>KSQVKIRFFTREKDELLHVQDTPMYAPISLKRYGLSEIVNHLLGSEKPVPFDFLIEGELLRTSLHDYLTKKGLSSEASLN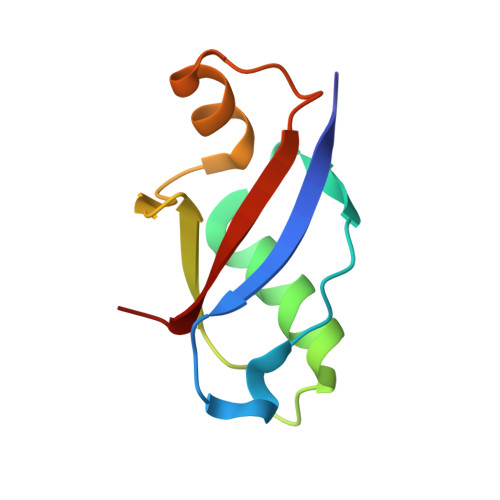VEYTRAIL[2x]>GSALEKVPVEEYLVHALQGSVSSGQAHSLASLAKTWSSGSAKLQRLGPETEDNEGVLLTEKLKPVDYEYREEVHWMTHQPRVGRGSFGEVHRMKDKQTGFQCAVKKVRLEVFRVEELVACAGLSSPRIVPLYGAVREGPWVNIFMELLEGGSLGQLIKQMGCLPEDRALYYLGQALEGLEYLHTRRILHGDVKADNVLLSSDGSRAALCDFGHALCLQPDGLGKSLLTGDYIPGTETHMAPEVVMGKPCDAKVDIWSS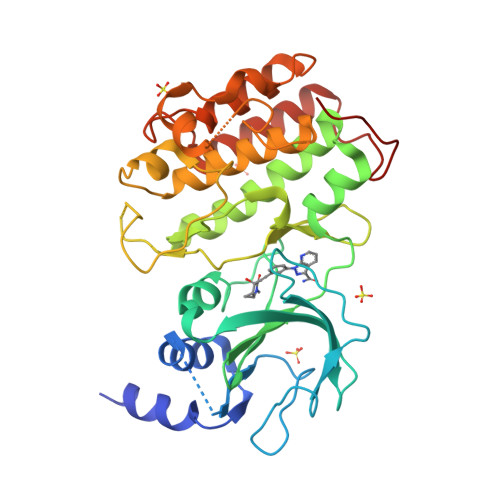CCMMLHMLNGCHPWTQYFRGPLCLKIASEPPPIREIPPSCAPLTAQAIQEGLRKEPVHRASAMELRRKVGKALQEVGGLKSPWKGEYKEPRGNS[2x]> RSPIRRSNYTPRNEKGLEGVIELQLNVVSDYLHVGSGKYDVEVMRSVSDVKRLVEDYLSGGNKRIPNNVDQYFSMVAFLMVRNKDNVVIPGSTIKGMVRSRLELSVPGSCYIVTGHSTSSSAVYKRIFNPDPNRGSDRFDVNKFPQVCPVCDLLGNMGLASRVSLSDFVMTSGKV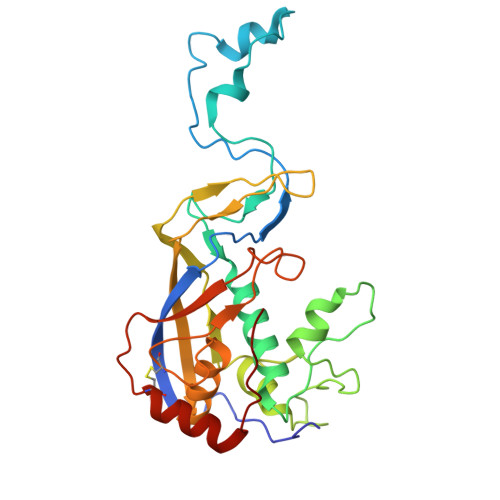DYVNVKGRDYEVVTKGSIFAGKVLYKSLKPVEIGMLLYGFGFVKDCNGSKVMLLGRFKFSDKRFGRVKFSLKTPIADCNKLVSDFVKQFNPRYINEE>[2x]MVEMGRREEMIAKIKELMLQPERIRNIGIAAHIDHGKTTLSDNLLAGAGMISEELAGKQLVLDFDEQEQARGITINAANVSMVHNYEGKDYLINLIDTPGHVDFGGDVTRAMRAIDGVIIVVDAVEGVMPQTETVVRQALREYVKPVLFINKVDRLIRELKLTPQQMMERFSKIIMDVNRLIQRYAPEEYKKKWMVKVEDGSVAFGSAYYNWALSVPFMKRTGVKFNEIIDLTLKGDNRTLRQKAPLHVVVLDMVVRHLPSPIEAQKYRIPH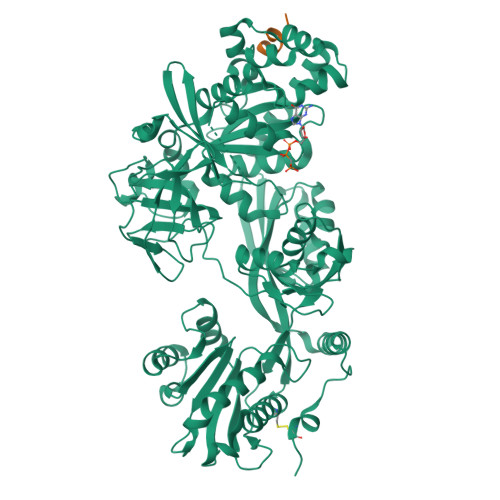LWEGDISSDIGQAMLNCDPKGKMVMVVTKIIIDKHAGEVATGRVWSGTVKSGQEVYLINTKRKARIQQVGIYMGPERINMEAVPAGNIVAVTGLRDAMAGETVAEEQIEPFEALHYVSEPVVTVAIEAKNVKDLPRLIEALRQLAKEDPTLHVKIDEETGQHLLSGMGELHLEVKLYKLKKDWGIDIEVSEPIVVYRESITKSSPMVEGKSPNRHNRFYIVVEPMPDEIYNAIKEGIIPEGRVKNPKEVAKKLAELGMDYEIARGIVDIYNGNMFIDNTKGVQYLNEVMDLLIDGFHQAMDEGPLAREPVMKVIVRLLDAQVHEDNVHRGPAQIYPAIRTAIHCAMMKSNPVLYEPYQKVIINIPYEYMGAVSREITQRRGQLVDMKQEGEVMTIIAEAPVAEMFGFAGSIRSATSGRALWSTEHAGFKRVPNELAQQIIRQIRQRKGLDPNPPTEKDVCPLFLEHHHHHH;>[2x]EALAGLSALFG>[2x]GRRGVL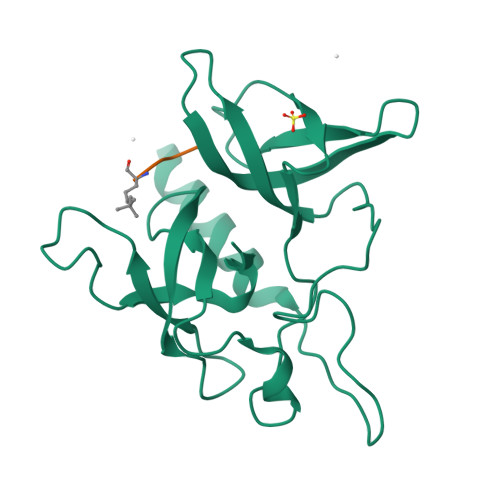MTLLQQSAMTLPLWIGKPGDKPPPLCGAIPASGDYVARPGDKVAARVKAVDGDEQWILAEVVSYSHATNKYEVDDIDEEGKERHTLSRRRVIPLPQWKANPETDPEALFQKEQLVLALYPQTTCFYRALIHAPPQRPQDDYSVLFEDTSYADGYSPPLNVAQRYVVACKEPKKK;>ARTXQTARKS[2x]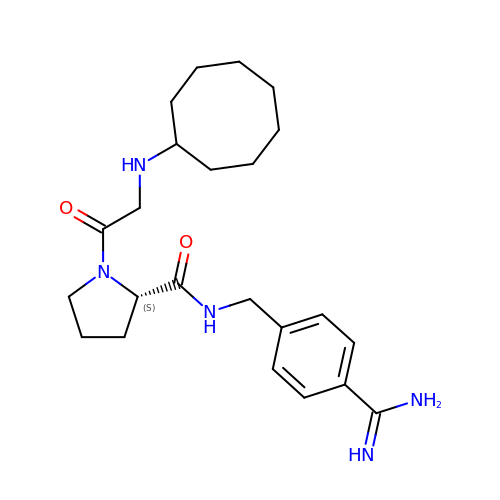N-cyclooctylglycyl-N-(4-carbamimidoylbenzyl)-L-prolinamide | C23 H35 N5 O2 | MMLOIDMSBRJZAE-FQEVSTJZSA-N> GSGGGGGSTQLNLRSLLVNPEGPTLMRLNSVQSSERPLFLVHPIEGSTTVFHSLASRLSIPTYGLQCTRAAPLDSIHSLAAYYIDCIRQVQPEGPYRVAGYSYGACVAFEMCSQLQAQQSPAPTHNSLFLFDGSPTYVLAYTQSYRAKLTPGCEAEAETEAICFFVQQFTDMEHNRVLEALLPLKGLEERVAAAVDLIIKSHQGLDRQELSFAARSFYYKLRAAEQY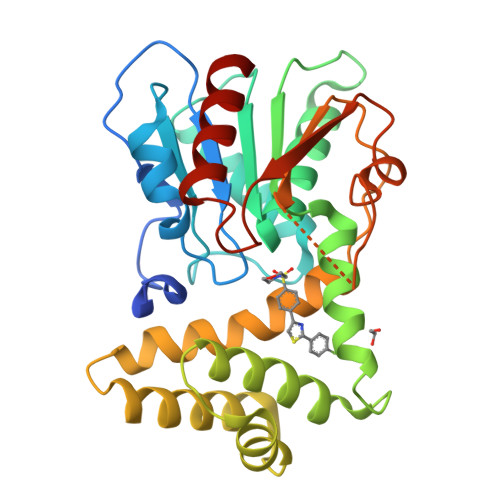TPKAKYHGNVMLLRAKTGGAYGEDLGADYNLSQVCDGKVSVHVIEGDHRTLLEGSGLESIISIIHSSLAEH>MERMQGEAEGDHLER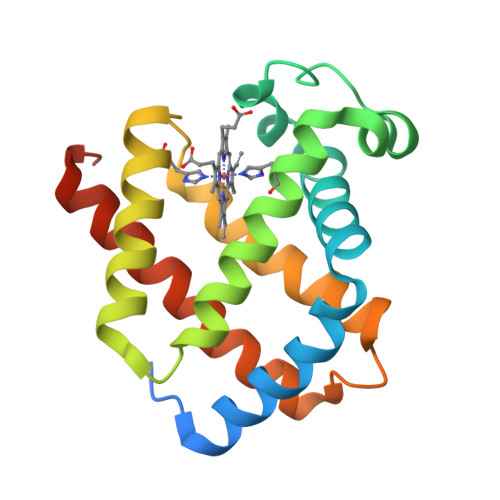PSPLTDKERVMIQDSWAKVYENSDDTGVAILVRLFVNFPSSRQYFSQFKHIEEPEELERSAQLRKHANRVMNGLNTLVESLDNSEKVASVLKLLGKAHALRHKVEPVYFKILSGVILEVLGEAFSEVVTPEVAAAWTKLLATIYSGINAVYEEVGWSKHSSSSG[2x]> MRVLVTGGSGYIGSHTCVQLLQNGHDVIILDNLCNSKRSVLPVIERLGGKHPTFVEGDIRNEALMTEILHDHAIDTVIHFAGLKAVGESVQKPLEYYDNNVNGTLRLISAMRAAN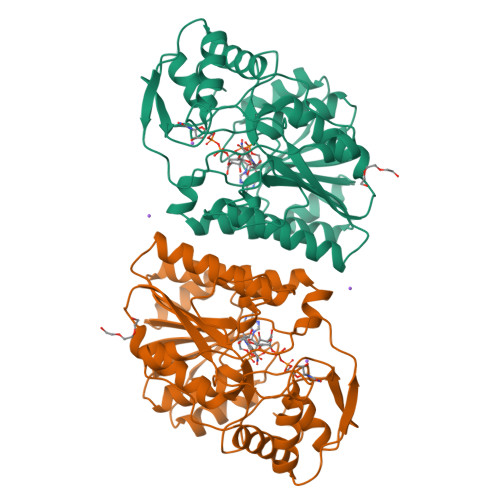VKNFIFSSAATVYGDNPKIPYVESFPTGTPQSPFGKSKLMVEQILTDLQKAQPDWSIALLRYFNPVGAHPSGDMGEDPQGIPNNLMPYIAQVAVGRRDSLAIFGNDYPTEDGTGVRDYIHVMDLADGHVVAMEKLANKPGVHIYNLGAGVGNSVLDVVNAFSKACGKPVNYHFAPRREGDLPAYWADASKADRELNWRVTRTLDEMAQDTWHWQSRHPQGYPD>APDTSVSNKQNFSTDVIYQIFTDRFSDGNPANNPTGAAFDGSCTNLRLYCGGDWQGIINKINDGYLTGMGITAIWISQPVENIYSVINYSGVNNTAYHGYWARDFKKTNPAYGTMQDFKNLIDTAHAHNIKVIIDFAPNHTSPASSDDPSFAENGRLYDNGNLLGGYTNDTQNLFHHYGGTDFSTIENGIYKNLYDLADLNHNNSSVDVYLKDAIKMWLDLGVDGIRVDAVKHMPFGWQKSFMATINNYKPVFTFGEWFLGVNEISPEYHQFANESGMSLLDLRFAQKARQVFRDNTDNMYGLKAMLEGSEVDYAQVNDQVTFIDNHDMERFHTSNGDRRKLEQALAFTLTSRGVPAIYYGSEQYMSGGNDPDNRARLPSFSTTTTAYQVIQKLAPLRKSNPAIAYGSTHERWINNDVIIYERKFGNNVAVVAINRNMNTPASITGLVTSLPRGSYNDVLGGILNGNTLTVGAGGAASNFTLAPGGTAVWQYTTDATTPIIGNVGPMMAKPGVTITIDGRGFGSGKGTVYFGTTAVTGADIVAWEDTQIQVKIPAVPGGIYDIRVANAAGAASNIYDNFEVLTGDQVTVRFVINNATTALGQNVFLTGNVSELGNWDPNNAIGPM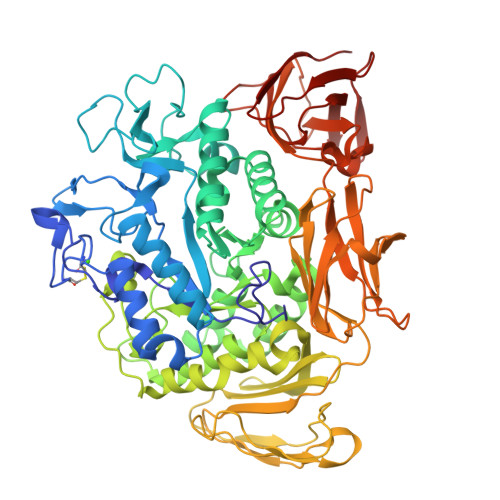YNQVVYQYPTWYYDVSVPAGQTIEFKFLKKQGSTVTWEGGANRTFTTPTSGTATVNVNWQP[2x]>[6x]PGEDRFKPVVPWPHVEGVEVDLESIRRINKAKNEQEHHAGGDSQKDIMQRQYLTFKPQTFTYHDPVLRPGILGNFEPKEPEPPGVVGGPGEKAKPLVLGPEFKQAIQASIKEFGFNMVASDMISLDRSVNDLRQEECKYWHYDENLLTSSVVIVFHNEGWSTLMRTVHSVIKRTPRKYLAEIVLIDDFSNKEHLKEKLDEYIKLWNGLVKVFRNERREGLIQARSIGAQKAKLGQVLIYLDAHCEVAVNWYAPLVAPISKDRTICTVPLIDVINGNTYEIIPQGGGDEDGYARGAWDWSMLWKRVPLTPQEKRLRKTKTEPYRSPAMAGGLFAIE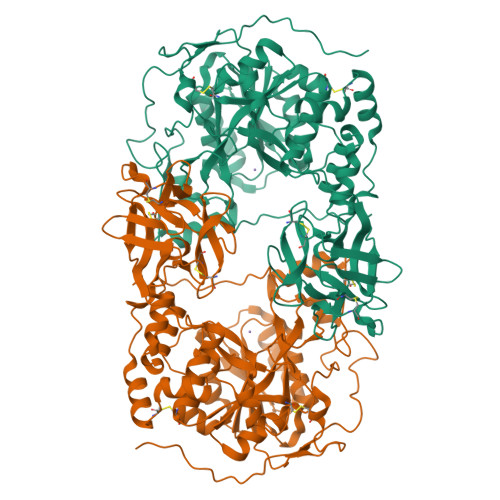REFFFELGLYDPGLQIWGGENFEISYKIWQCGGKLLFVPCSRVGHIYRLEGWQGNPPPIYVGSSPTLKNYVRVVEVWWDEYKDYFYASRPESQALPYGDISELKKFREDHNCKSFKWFMEEIAYDITSHYPLPPKNVDWGEIRGFETAYCIDSMGKTNGGFVELGPCHRMGGNQLFRINEANQLMQYDQCLTKGADGSKVMITHCNLNEFKEWQYFKNLHRFTHIPSGKCLDRSEVLHQVFISNCDSSKTTQKWEMNNIHSV> KHSLPDLPYDYGALEPHINAQIMQLHHSKHHAAY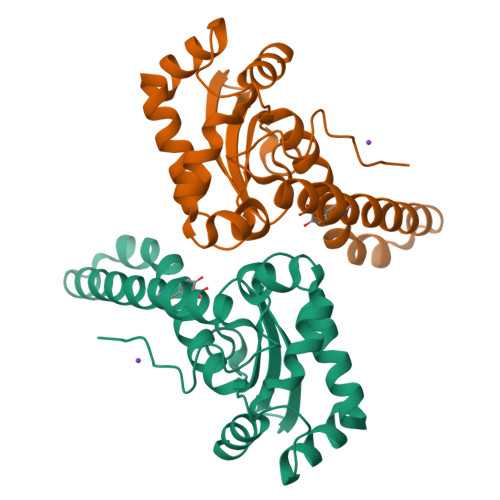VNNLNVTEEKYQEALAKGDVTAQIALQPALKFNGGGHINHSIFWTNLSPNGGGEPKGELLEAIKRDFGSFDKFKEKLTAASVGVQGSGWGWLGFNKERGHLQIAACPNQDPLQGTTGLIPLLGIDVWEHAYYLQYKNVRPDYLKAIWNVINWENVTERYMACKK> MAPVRS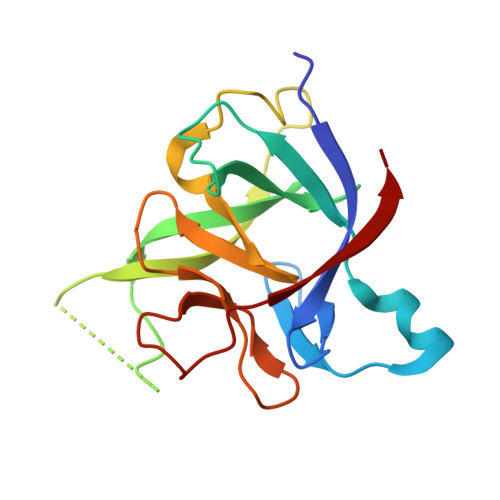LNCTLRDSQQKSLVMSGPYELKALHLQGQDMEQQVVFSMSFVQGEESNDKIPVALGLKEKNLYLSCVLGYIDTNNDGWIEGDELYPTLQLESVDPKNYPKKKMEKRFVFNKIEINNKLEFESAQFPNWYISTSQAENMPVFLGGTKGGQDITDFTMQFVSS> GAMDYSLVKALQTAQQNFVISDPSIPDNPIVYASQGFLTLTGYALSEVLGRNCRFLQGPETDPKAVEKVRKGLERGEDTTVVLLNYRKDGSTFWNQLFIAALRDGEGNVVNYLGVQCKVSEDYAKAFLKN;> GAMDYSLVKALQTAQQNFVISDPSIPDNPIVYASQG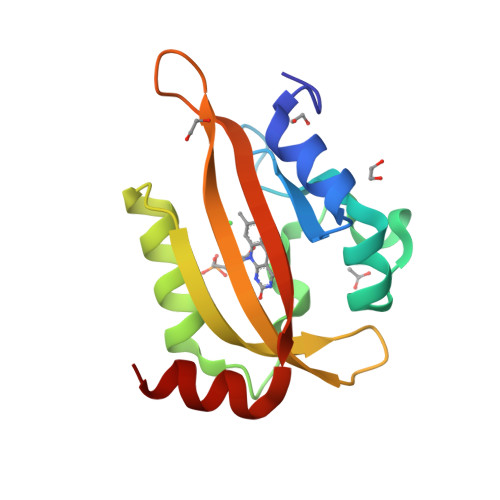FLTLTGYALSEVLGRNCRFLQGPETDPKAVEKVRKGLERGEDTTVVLLNYRKDGSTFWNQLFIAALRDGEGNVVNYLGVQCKVSEDYAKAFLKNEEN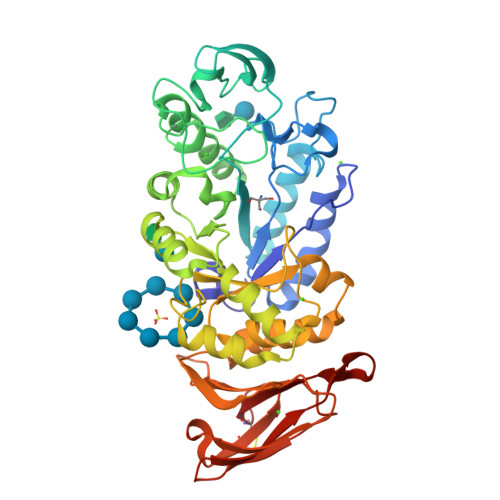> AKYSELEKGGVIMQAFYWDVPSGGIWWDTIRQKIPEWYDAGISAIWIPPASKGMGGAYSMGYDPYDFFDLGEYDQKGTVETRFGSKQELVNMINTAHAYGMKVIADIVINHRAGGDLEWNPFVNDYTWTDFSKVASGKYTANYLDFHPNELHAGDSGTFGGYPDICHDKSWDQYWLWASQESYAAYLRSIGIDAWRFDYVKGYAPWVVKDWLNWWGGWAVGEYWDTNVDAVLNWAYSSGAKVFDFALYYKMDEAFDNKNIPALVSALQNGQTVVSRDPFKAVTFVANHDTDIIWNKYPAYAFILTYEGQPTIFYRDYEEWLNKDKLKNLIWIHENLAGGSTDIVYYDNDELIFVRNGYGDKPGLITYINLGSSKAGRWVYVPKFAGACIHEYTGNLGGWVDKYVYSSGWVYLEAPAYDPANGQYGYSVWSYCGVG>[2x]GSHMYIGPEVPKEDLIWQDPLPQPIYNPTEQDIIDLKFAIADSGLSVSELVSVAWASASTFRGGDKRGGANGARLALMPQRDWDVNAAAVRALPVLEKIQKESGKASLADIIVLAGVVGVEKAASAAGLSIHVPFAPGRVDARQDQTDIEMFELLEPIADGFRNYRARLDVSTTESLLIDKAQQL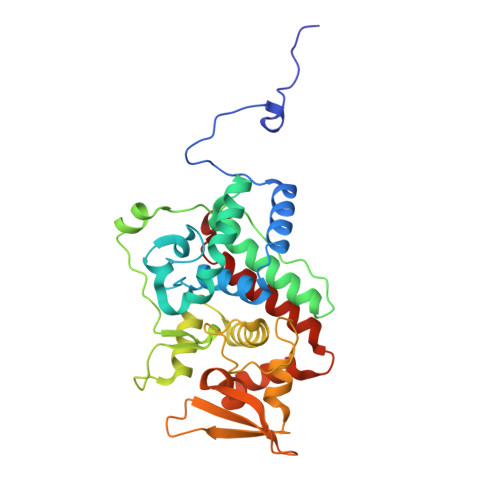TLTAPEMTALVGGMRVLGANFDGSKNGVFTDRVGVLSNDFFVNLLDMRYEWKATDESKELFEGRDRETGEVKFTASRADLVFGSNSVLRAVAEVYASSDAHEKFVKDFVAAWVKVMNLDRFDLL> GPKQKIVIKATMSNAKSRAQAMVLASKANGVGSVGITGDLKDQLEVVGVGIDIACLVRCLRKKLRYAEIVKVEEVKDK;> MQNEYLDAKKHGIDLSRE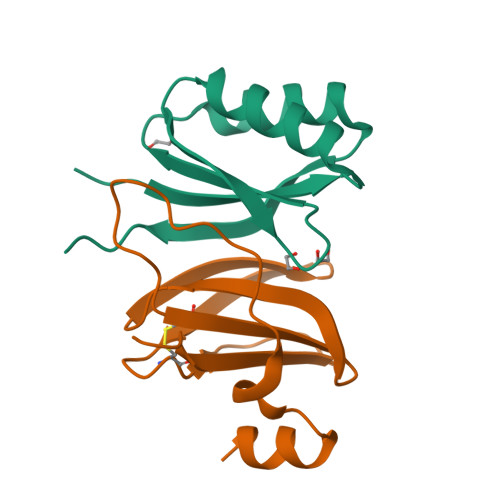RAPNFVDHPGIPPSDCFWFLYKNYVRQDAGVCQSDWSFDMKIGQYWVTIHTDEGCRLSGIIPAGWLILGIKRLGF>CFAKGTNVLMADGSIECIENIEVGNKVMGKDGRPREVIKL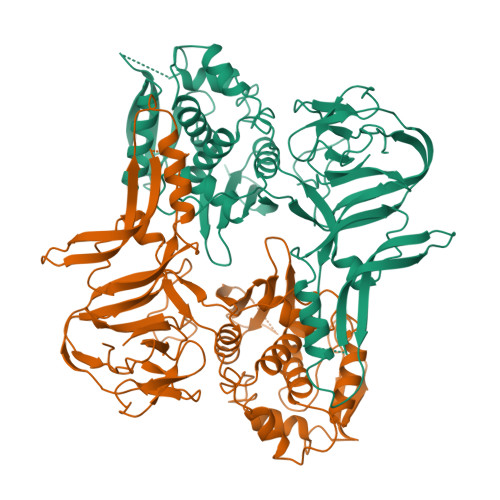PRGRETMYSVVQKSQHRAHKSDSSREVPELLKFTCNATHELVVRTPRSVRRLSRTIKGVEYFEVITFEMGQKKAPDGRIVELVKEVSKSYPISEGPERANELVESYRKASNKAYFEWTIEARDLSLLGSHVRKATYQTYAPILYENDHFFDYMQKSKFHLTIEGPKVLAYLLGLWIGDGLSDRATFSVDSRDTSLMERVTEYAEKLNLCAEYKDRKEPQVAKTVNLYSKVVRGNGIRNNLNTENPLWDAIVGLGFLKDGVKNIPSFLSTDNIGTRETFLAGLIDSDGYVTDEHGIKATIKTIHTSVRDGLVSLARSLGLVVSVNAEPAKVDMNGTKHKISYAIYMSGGDVLLNVLSKCAGSKKFRPAPAAAFARECRGFYFELQELKEDDYYGITLSDDSDHQFLLANQVVVHN[2x]Ferrous GLB-1 binds O2 with a high affinity and is pentacoordinated in the absence of exogenous heme ligands. The tertiary structure of GLB-1* conforms to the three-over-three α-helical sandwich of the classical globin fold, where the seven/eight helices building up the globin fold are conventionally labelled, A, B..., H, according to their sequential order (topological sites are numbered sequentially within each helix;). The GLB-1* heme distal site resembles that of A. suum Hb, with TyrB10 directly stabilizing the O2 molecule and GlnE7 making a hydrogen bond with the B10 residue. Taken together, the observed functional data suggest for GLB-1 a putative role in vivo related to O2 binding, NO scavenging or O2 storage.

The structure of GLB-1* (bearing the Cys(127)GH2 → Ser mutation to avoid protein aggregates during crystallization) was solved by MAD methods based on the anomalous signal of the heme iron atom. Diffraction data were collected at three wavelengths at the ID29 ESRF beamline (Grenoble, France), for the tetragonal P43212 form (one GLB-1* molecule per asymmetric unit). Refinement of the crystal structure (at 1.5 Å resolution) converged at a general Rfactor value of 16.3% (Rfree of 20.1%), with ideal stereochemical parameters. The final model contains 1,305 protein atoms (residues 2-159), 1 heme, 1 dioxygen molecule and 202 ordered solvent atoms (2 of them in alternate sites). In the high resolution tetragonal crystal form the crystallographic two-fold axis gives rise to a GLB-1* homodimer, whose 945 Å2 association interface is mostly built by residues belonging to the E- and F helices (residues 72-83, and 87-101 respectively), and to the AB (residues 20-25) and EF (residues 84-86) corners of both chains. Stabilization of the heme group within the GLB-1* fold occurs through 95 van der Waals contacts (≤ 4.0 Å); moreover, salt links are present between residue Arg(65)E3 and heme A-propionate, and between residue Arg(100)F7 and heme D-propionate. The proximal His(101)F8 residue is properly coordinated to the heme-Fe atom (2.06 Å coordination bond), and is fully staggered relative to the porphyrin pyrrole N-atoms, allowing in principle a short Fe--HisF8 coordination bond, and in-plane location of the Fe atom. The HisF8 staggered orientation is defined by a strong hydrogen bond (2.83 Å) of His(101)F8 ND1 atom to the carbonyl O atom of residue Thr(97)F4. Tyr(35)B10 and Gln(69)E7 are the only polar residues in the heme distal site, which is essentially lined by aromatic residues (Phe(34)B7, Phe(38)B11, Phe(49)C6, Phe(66)E4, Ile(73)E11, and Phe(114)G8). Likely related to the overall apolarity, but also to the steric constraints posed by the above mentioned residues, no water molecules are observed in the heme distal site.

> MSMNRQEISDLCVKSLEGRMVGTEAQNIENGNAFYRYFFTNFPDLRVYFKGAEKYTADDVKKSERFDKQGQRILLACHLLANVYTNEEVFKGYVRETINRHRIYKMDPALWMAFFTVFTGYLESVGSLNDQQKAAWMALGKEFNAESQTHLKNSNLPHV> MAARTDNSIVVNAPFELVWDVTNDIEAWPELFSEYAEAEILRQDGDGFDFRLKTRP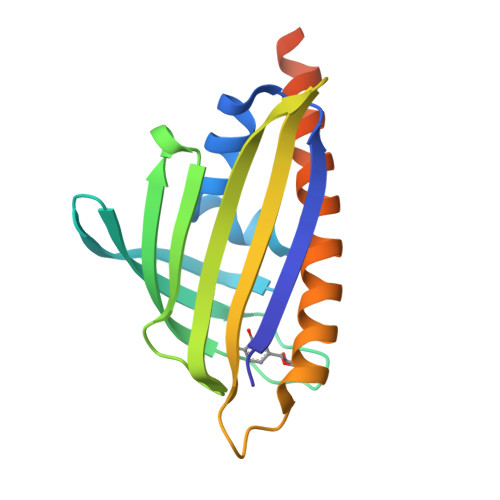DANGRVWEWVSHRVPDKGSRTVRAHRVETGPFAYMNLHWTYRAVAGGTEMRWVQEFDMKPGAPFDNAHMTAHLNTTTRANMERIKKIIEDRHREGQRTPASVLPTELHAQQLL> MKVGQDKVVTIRYTLQVEGEVLDQGELSYLHGHRNLIPGLEEALEGREEGEAFQAHVPAEKAYGPHDPEGVQVVPLSAFPEDAEVVPGAQFYAQDMEGNPMPLTVVAVEGEEVTVDFNHPLAGKDLDFQVEVVKVREATPEELLHGHAHPSGHHHHHH;>VGSNSYPHKYNNYEGX[2x]

Peptidyl-prolyl isomerases (PPIases) catalyze cis/trans isomerization of peptidyl-prolyl bonds, which is often rate-limiting for protein folding. SlyD is a two-domain enzyme containing both a PPIase FK506-binding protein (FKBP) domain and an insert-in-flap (IF) chaperone domain. In order to improve our understanding of the mechanism of SlyD and of FKBPs in general, we set out to analyze the kinetics, energetics, and structural basis for substrate binding and inhibition of SlyD from Thermus thermophilus (TtSlyD) using 15-residue-long unmodified peptides, which we reasoned would be better mimics of natural unfolded protein substrates than the traditionally used 4-nitroanilide tetrapeptides. In total, we obtained five structures of TtSlyDFL and three of TtSlyDΔIF at a maximum resolution of up to 1.4 Å.

For the T1 peptide, a single-site model was sufficient to describe binding to TtSlyDFL, and the affinity was found to be much lower (KD = 158 μM) than for the S2 and S3 peptides, which is explained primarily by an increase in unfavorable binding entropy. A peptide is bound to the IF domain in four structures: TtSlyDFL:S2, TtSlyDFL:S2-W23A, TtSlyDFL:S2-plus, and TtSlyDFL:T1. Interestingly, although the binding mode is variable, three aspects are shared for all structures: (i) the peptides bind to the β8–β9 hairpin through β-strand augmentation with two to four hydrogen bonds, (ii) the peptides generally insert two hydrophobic side chains into the binding groove as detailed above, and (iii) peptide binding does not perturb the hydrophobic groove. Interestingly, the proline residues of the peptides bound to the IF domains are all in the trans conformer—with the possible exception of the S2 peptide bound to molecule B in the TtSlyDFL:S2 structure, where P29S2 could be in cis configuration —and in most cases do not form direct interactions with the IF domain. The TtSlyDFL:T1 and TtSlyDΔIF:S3 structures both show alternative binding modes. The T1 peptide adopts a reverse orientation as compared to the S2 and S2-W23A peptides, and forms only few interactions with the FKBP domain. The non-canonical binding modes agree well with the weaker affinities of these peptides, but it is unclear if they mimic any physiologically relevant interactions.> GVENAEKGVTENTDATADFVAQPVYLPENQTKVAFFYDRSSPIGAFAVKSGSLESGFAPFSNKACPNSVILTPGPQFDPAYDQLRPQRLTEIWGNGNEETSEVFPLKTKQDYSFCLFSPFVYYKCDLEVTLSPHTSGAHGLLVRWCPTGTPTKPTTQVLHEVSSLSEGRTPQVYSAGPGTSNQISFVVPYNSPLSVLPAVWYNGHKRFDNT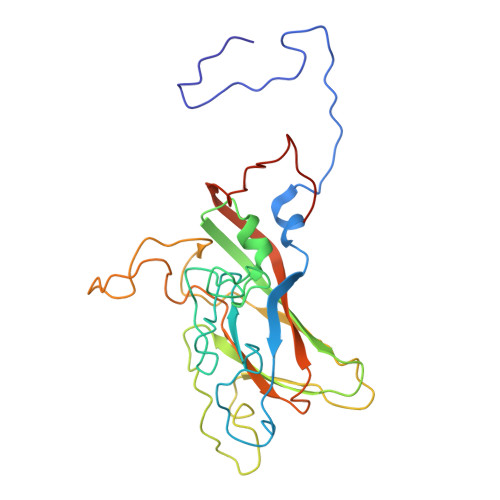GDLGIAPNSDFGTLFFAGTKPDIKFTVYLRYKNMRVFCPRPTVFFPWPTSGDKIDMTPRAGVLMLE> SLEKRAQLCQPDAHGVRRFNGRP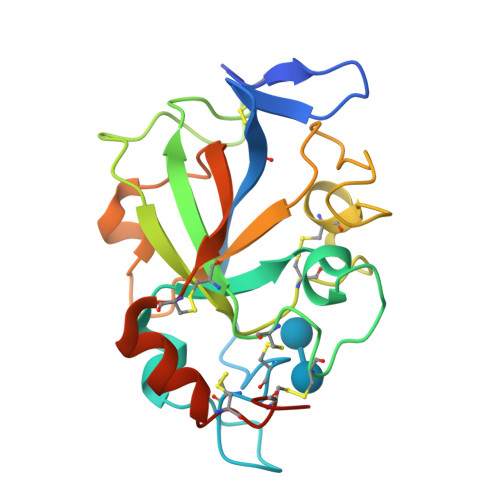CASTTRYVDGHKGACGCGQKGSDTPFPWNLQKHVTAPSERYFDDGGSNLWCGKNCGKCVRLTPTGGFVPGKGGAPPNHNPVVFMVTNACPINGNEEWCGISGKPGTNHVNSHGYEVHFALQDQVGQVEALHWDNPEVTWEEVPCPGDLQANYQQCECHNSDHHHHHH>MFRVGILTVSDKGFRGERQDTTHLAIREVLAGGPFEVAAYELVPDEPPMIKKVLRLWADREGLDLILTNGGTGLAPRDRTPEATRELLDREVPGLAELMRLVGLRKTPMAALSRGVAGVRGRTLILNLPGSPKGARESLEAVLPVLPHALSLVTGKPWKEGHHE[3x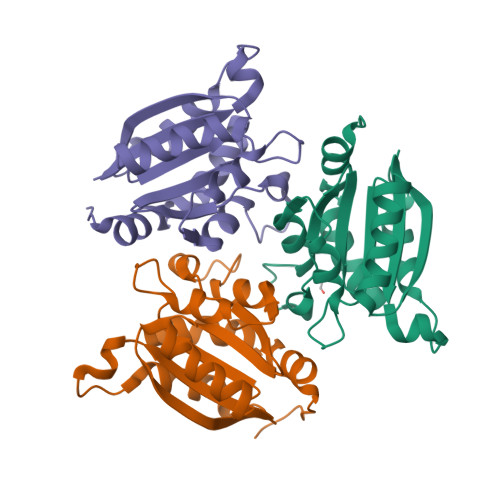]4-(2-{(4M)-4-[(6M)-6-(2,5-dimethoxyphenyl)pyridin-3-yl]-1H-1,2,3-triazol-1-yl}ethyl)-N-{[1-(methoxymethyl)cyclopropyl]methyl}-N-methylbenzamide | C31 H35 N5 O4 | 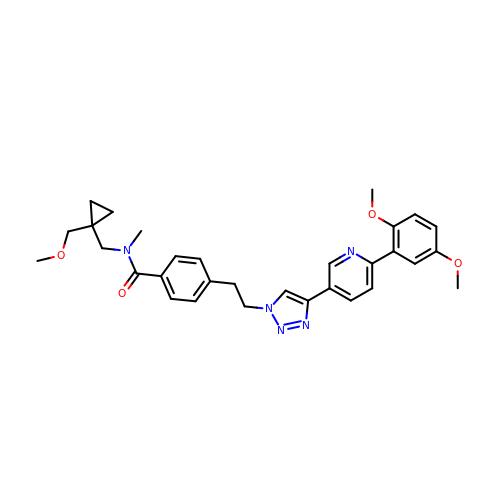MGTHESHOEDYGFD-UHFFFAOYSA-N>[2x]AEVNDPRVGFVAVVTFPVDGPAT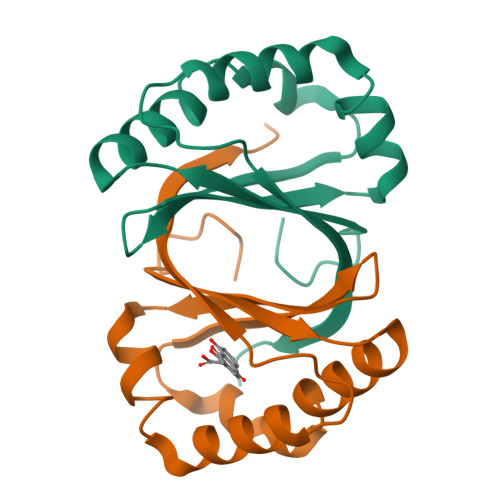QHKLVELATGGVQEWIREVPGFLSATYHASTDGTAVVNYAQWESEQAYRVNFGADPRSAELREALSSLPGLMGPPKAVFMTPRGAILPS> MSKFLKNRAVVNGLPVIKNPGKYQHCYLIEYEDSTNVKQTPTENKNKQQQGFPVYLFMMNPENITYNLPINYQEIAIPFTAKNQLNYSNGGNIVMTMSNLILDTMDEKRSLQPLIDRLIALREPTVKKGLKSHPKILAFKWGSNTFAPCVLTNISFDVTRWIDGYPTKAR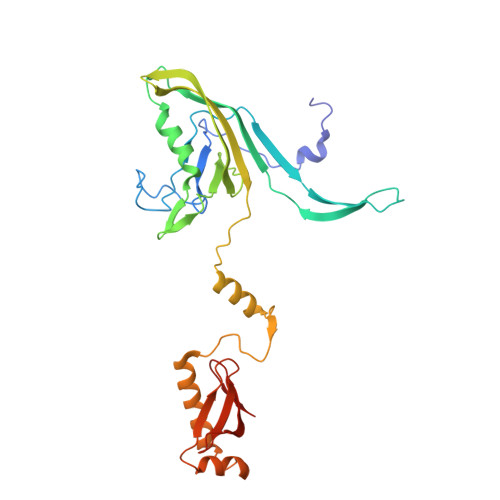VNMSLKEIQKPSSDSKALEEAKKKVKVETVQNGNLKKTLSEKQLIDGVKRVTEYLKKNISFQPRTIQNILSDPKSVIKIDKDTGQVSLFNGNGEFAALVGTYNGDIFSPSRQ> ALWQFNGMIKCKIPSSEPLLDFNNYGCYC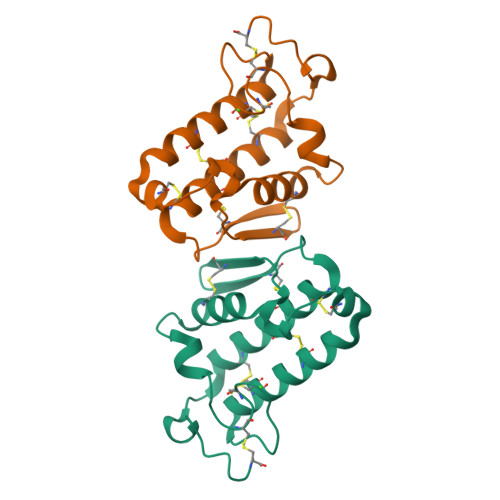GLGGSGTPVDDLDRCCQTHDNCYKQAKKLDSCKVLVDNPYTNNYSYSCSNNEITCSSENNACEAFICNCNRNAAICFSKVPYNKEHKNLDKKNC> 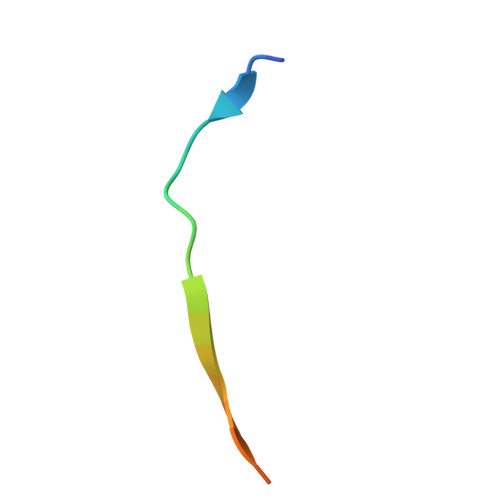MTKTYTAPTLVEYGGLERLT> AMALEARLEQASILKKVVDAIKDL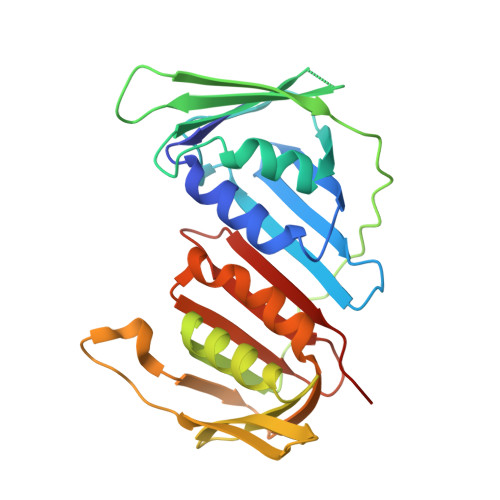VQDCNFDCNDSGIALQAMDNSHVALVSMMLKAEGFSPYRCDRNIALGVNLTSLTKVLRAAQNEDILTLKAEDAPDVLNLVFESSETDRISEYDLKLMDIDQEHLGIPETEYAATITMPSNEFKRITTDLMAMSESVTIEANKDGVKFSCQGDIGNGSVTLRQHTNVEKPNESIEIELSEPVSLTFSLKYLVNFCKASALSNTVKICLSNEVPLLVEYSLGGSSYLRFYLAPKIGDDE> MLYILNSAILPLKPGEEYTVKAKEITIQEAKELVTKEQFTSAIGHQATAELLSSILGVNVPMNRVQIKVTHGDRIL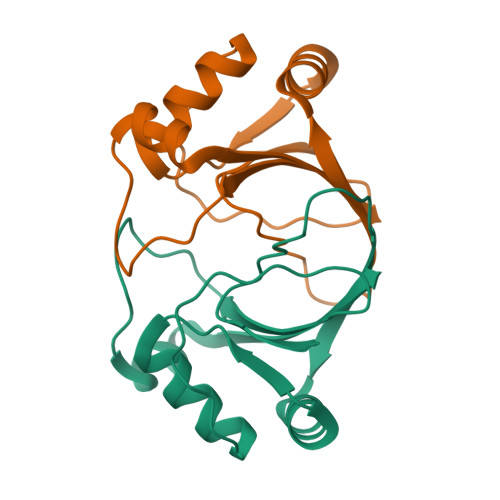AFMLKQRLPEGVVVKTTEELEKIGYELWLFEIQ> HKCDITLQEIIKTLNSLTEQKTLCTELTVTDIFAASKNTTEKETFCRAATVLRQFYSHHEKDTRCLGATAQQFHRHKQLIRFLKRLDRNLWGLAGLNSCPVKEANQSTLENFLERLKTIMREKYSKCSS;> FKVLQEPTC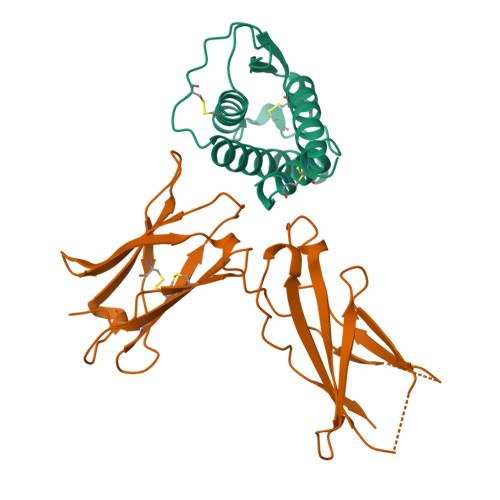VSDYMSISTCEWKMNGPTNCSTELRLLYQLVFLLSEAHTCIPENNGGAGCVCHLLMDDVVSADNYTLDLWAGQQLLWKGSFKPSEHVKPRAPGNLTVHTNVSDTLLLTWSNPYPPDNYLYNHLTYAVNIWSENDPADFRIYNVTYLEPSLRIAASTLKSGISYRARVRAWAQAYNTTWSEWSPSTKWHNSYREPFEQH> QGPLGSKLSEHLRYCDSILREMLSKKHAAYAWPFYKPVDAEALELHDYHDIIKHPMDLSTVKRKMD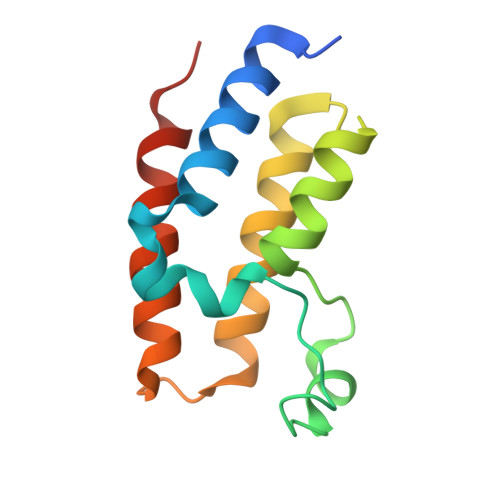GREYPDAQGFAADVRLMFSNCYKYNPPDHEVVAMARKLQDVFEMRFAKMPDEP>[4x]MDEESASRASVPASSDREGAEFTRLPVSWTVNPRDAANARAAWKTLSAYHRGKPKSSRKLHVVYVTFKDRPALEGYRERYDHILKNIQAYYADQMQANGFPPLTFQLDLDERGKLVIHDAYVDKPMSEMSVQSSGPVSREAARKVLASKGIDIEKEHVLVVCQLPDGVGPYYGGGFSHQGTGWTCDQEGLDPASFLDTEMMQGGRFKVTRGKNATIYIGGTAHELGHSFGLPHT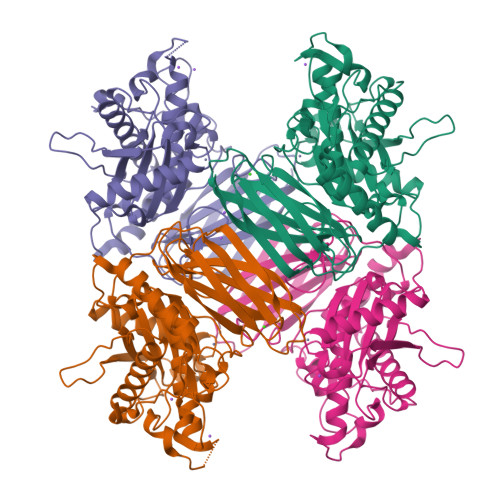GDGWNYPDAGASLMGHGNSTYGDELRHEGKGAYLAPTDALKLASVPLFNGVETELPADASFGRMLGKYVPGSFERLEAIPVKDGLRLKGRVHLTRPAYGIVAHLDPPGGSDYDSNAVGASLDEKGEFDLTICRPGYKGGFIEMRVAVLNCDSTRSMITLPVWMDARGTKAPSLAQIVYFGDVQNLWIRGRTEEARKALAEVERRHGSRSEVKEWLPVWKRALGRQEPALEVVPAQIPAATASISLNDCKPSV>GQESAEFRPAELAGIWQLCHYVSEIPDVPGILKPSNTFKVLSDDGRIVNFTMIPGKD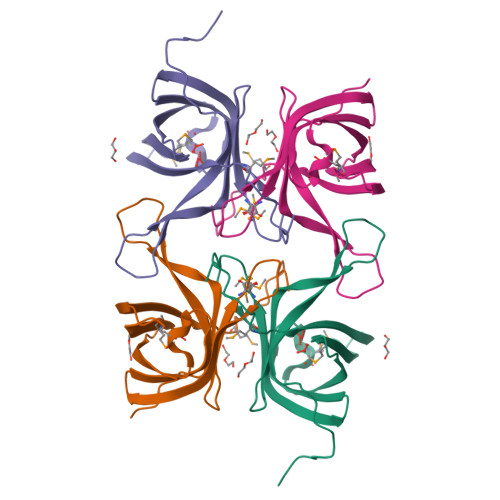AIITGYGTYQQLTDNSYKESIEKNIHLPMLDHKDNILEFEIGDDGVMYLKYFIAKDLNGNELNTWFHETWKRVGMPAKFPEDLVR[4x]>[4x]MAHHHHHHMAIRKILYLPDERLRKIAKPVETFDESLQTLINDMFDTMYDARGVGLAAPQIGVSLRLSVIDIVGDKKEQIVIVNPEIVSSHGEKEFEEGCLSVPGAY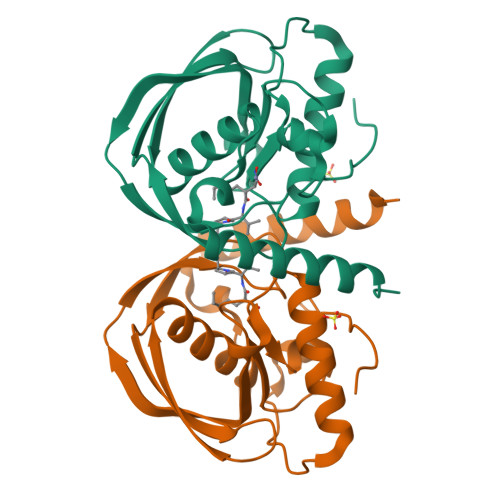DTVVRAEKVTVKALDRFGKPFEITGEGLLAECLQHEIDHMNGKLFVDMLSPLKRMMARRKLDKFKRLQARKP> MNVGINWSGQRELPCINQLFLTRDIDFVELLIDNFLTTDVDSIKAFLAGRPCAFHIMNSQFLHKDERELLAMAKIINKLIHSLQPIYISDHIGKFYHRGQALPQMLEVDYGLQTHSTIKKVKAWSSLLDGKLLLENYPSIFPQDMSQIDFFKRILEETYCGLLFDISNAFIAEVNIKQSRTSWFDLIKHCQHFHIAGFENAPDNQFLVDTHSQCIEEPV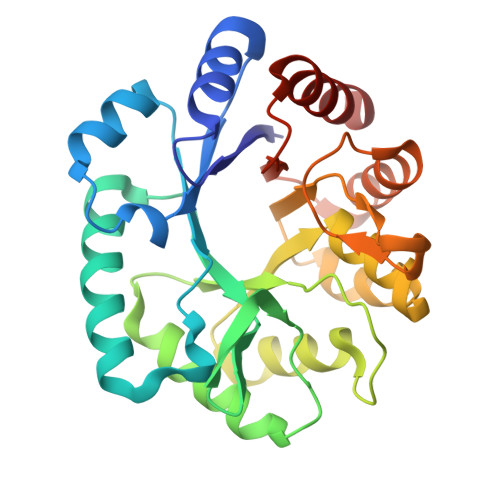LSFLQEVNNATSIATISVERDENFDVSDWALDIDNVRNRVS Here, we report the crystal structures of PhoExo I, which shares 76% amino acid sequence identity with PfuExo I. In this study, we determined three substrate-free structures of PhoExo I and four structures of PhoExo I in complexes with ssDNAs. PhoExo I forms a trimer in solution similar to PfuExo I. The 3′-5′ exonuclease assay of PhoExo I showed that PhoExo I cleaved an ssDNA from its 3′-end at every two nucleotides, and the cleavage stopped at the third to fifth nucleotide from the 5′-end. PhoExo I is predicted to utilize a DEDE (RNase HIII)-type catalytic motif for the hydrolysis of ssDNA. PhoExo I is a novel RNase H superfamily protein.

In this study, we determined three substrate-free PhoExo I structures using three crystals with different unit-cell parameters (crystals 1–3). Crystal 3 contained two PhoExo I protomers in the asymmetric unit. In crystal 3, each protomer of PhoExo I formed a trimer with symmetrically related proteins that were generated by the crystallographic 3-fold axis. Because the structures of PhoExo I in crystals 1 and 2 were partially disordered, we mainly used the structure of PhoExo I in crystal 3 for the images, unless otherwise stated. In the structures of PhoExo I, each PhoExo I protomer binds one Mg2+ ion among the β1 strand of the large β sheet, the α1 helix, the β4–β5 loop and the longest α4 helix. The Mg2+ ion is coordinated by Asp7, Asp80 and four water molecules in an octahedral manner. Because PhoExo I requires Mg2+ ions for its 3′-5′ exonuclease activity, PhoExo I is predicted to catalyse the hydrolysis of an ssDNA around this magnesium-binding site. PhoExo I forms a hexagram-like trimeric structure using the η3 helix, the N-terminus of the α4 helix, the η4 helix and the β11–β12 loop. In addition, Glu210 and Glu224 of one protomer form two ion pairs with Lys32 of the other protomer. It is noteworthy that two arginine residues in each protomer, Arg191 and Arg219, are clustered at the centre of the PhoExo I trimer, and the positive charges of these residues are neutralized by the negative charge of Asp189, which prevents electrostatic repulsion at the 3-fold axis region of the trimer. In contrast, the binding of a Mg2+ ion near the A site was not observed in the PhoExo I structures.

>[2x]MRIVAADTGGAVLDESFQPVGLIATVAVLVEKPYKTSKRFLVKYADPYNYDLSGRQAIRDEIELAIELAREVSPDVIHLDSTLGGIEVRKLDESTIDALQISDRGKEIWKELSKDLQPLAKKFWEETGIEIIAIGKSSVPVRIAEIYAGIFSVKWALDNVKEKGGLLVGLPRYMEVEIKKDKIIGKSLDPREGGLYGEVKTEVPQGIKWELYPNPLVRRFMVFEITSKS pivalyl-coenzyme A | C26 H44 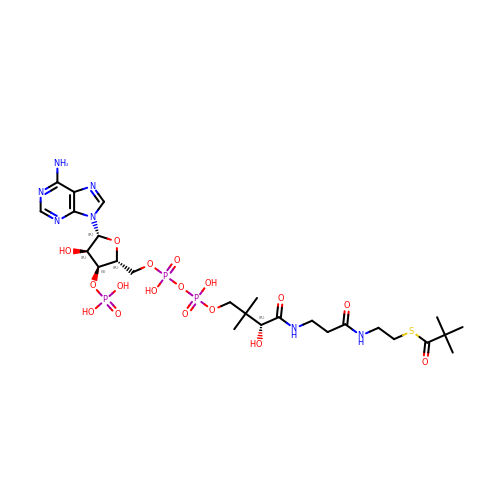N7 O17 P3 S | FCMKBHDFOPWWQK-NDZSKPAWSA-N> GPMSEAADVERVYAAMEEAAGLLGVACARDKIYPLLSTFQDTLVEGGSVVVFSMASGRHSTELDFSISVPTSHGDPYATVVE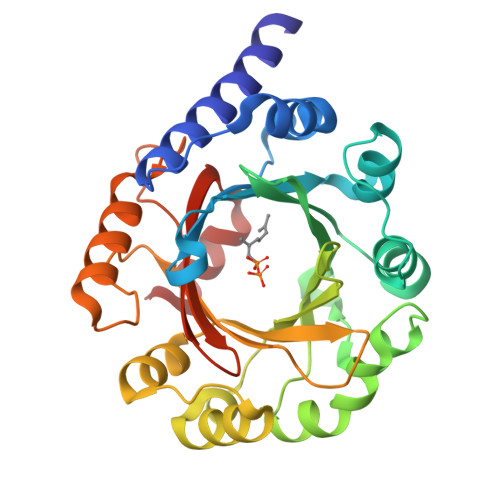KGLFPATGHPVDDLLADTQKHLPVSMFAIDGEVTGGFKKTYAFFPTDNMPGVAELSAIPSMPPAVAENAELFARYGLDKVQMTSMDYKKRQVNLYFSELSAQTLEAESVLALVRELGLHVPNELGLKFCKRSFSVYPTLNWETGKIDRLCFAVISNDPTLVPSSDEGDIEKFHNYATKAPYAYVGEKRTLVYGLTLSPKEEYYKLGAYYHITDVQRGLLKAFDSLED> GATEPGSQYQQQAEAG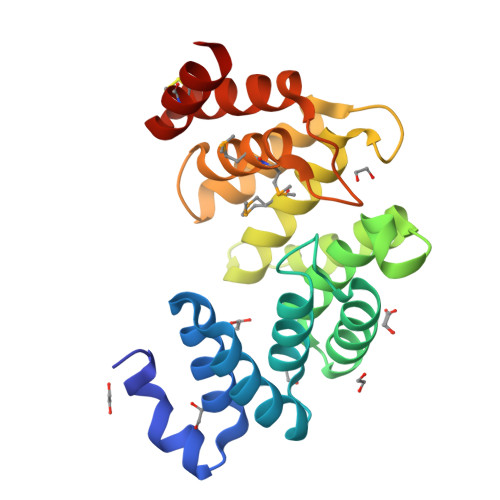DRRAQYYLADTWVSSGDYQKAEYWAQKAAAQGDGDALALLAQLKIRNPQQADYPQARQLAEKAVEAGSKSGEIVLARVLVNRQAGATDVAHAITLLQDAARDSESDAAVDAQMLLGLIYASGVHGPEDDVKASEYFKGSSSLSRTGYAEYWAGMMFQQGEKGFIEPNKQKALHWLNVSCLEGFDTGCEEFDRISKG> SLSDKDKDSIKAFWAKISPKAEDIGADALARMLTVYPQTKTYFSHW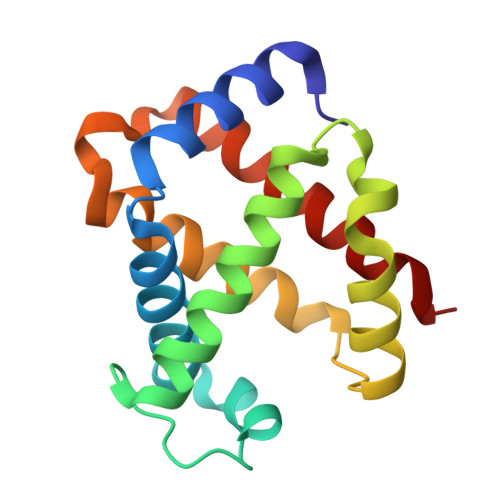KDLSPGSAPVKKHGKTVMGSVAEAVSKIDDLTNGLLTLSELHAFQLRVDPANFKILSHNLLVVLAQQFPNDFTPEVHVSMDKFLSLLSWSLSEKYR>[4x]EVVPSSALSEVSLRLLCHDDIDTVKHLCGDWFPIEYPDSWYRDITSNKKFFSLAATYRGAIVGMIVAEIKNRTKIHKEDGDILASNFSVDTQVAYILSLGVVKEFRKHGIGSLLLESLK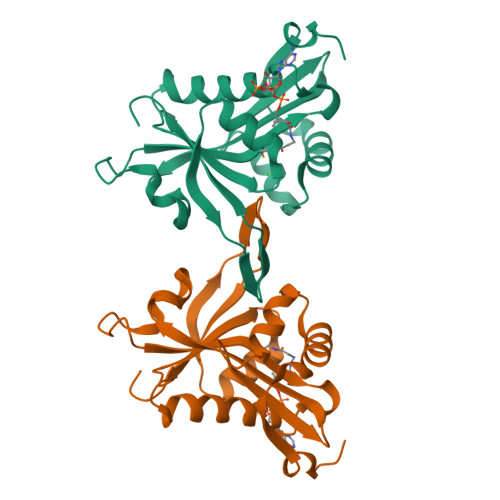DHISTTAQDHCKAIYLHVLTTNNTAINFYENRDFKQHHYLPYYYSIRGVLKDGFTYVLYINGG> SLAKRIIAALEVKDGRVVKGTNFENLRDSGDPVELGKFYSEIGIDELVFHDHTASVEKRKTMLELVEKVAEQIDIPFTVGGGIHDFETASELILRGADKVSINTAAVENPSLITQIAQTFGSQAVVVAIDAKRVDGEFMVFTYSGKKNTGILLRDWVVEVEKRGAGEILLTSIDRDGTKSGYDTEMIRFVRPLTTLPII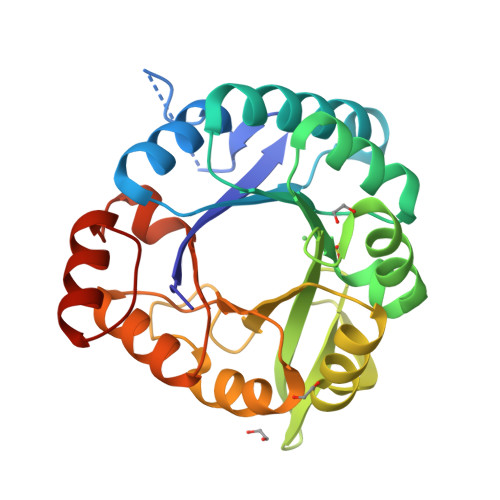ASGGAGKMEHFLEAFLAGADAALAASVFHFREIDVRELKEYLKKHGVNVRLEGL> MDLTVEPNLHSLITSTTHKWIFVGGKGGVGKTTSSCSIAIQMALSQPNKQFLLISTDPAHNLSDAFGEKFGKDARKVTGMNNLSCMEIDPSAALKDMNDMAVSRANNNGSDGQGDDLGSLLQGGALADLTGSIPGIDEALSFMEVMKHIKRQEQGEGETFDTVIFDTAPTGHTLRFLQLPNTLSKLLEKFGEITNKLGPMLNSFMGAGNVDISGKLNELKANVETIRQQFTDPDLTTFVCVCISEFLSLYETERLIQELISYDMDVNSIIVNQLLFAENDQEHNCKRCQARWKMQKKYLDQIDELYEDFHVVKMPLCAGEIRGLNNLTKFSQFLNKEYNPITDGKVIYELEDKEGLVPRGSLEHHHHH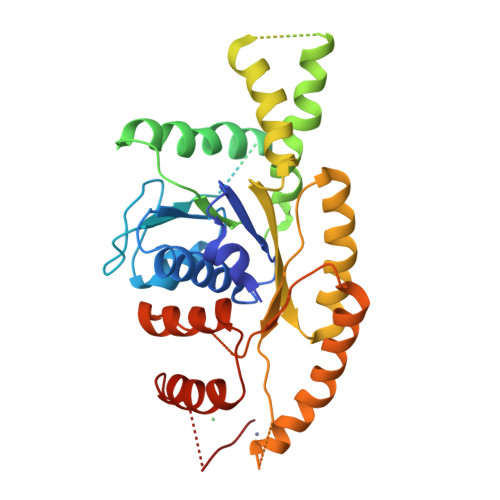H Human TNIK consists of serine–threonine kinase and scaffold domains2146. TNIK interacts directly with TCF4 and β-catenin, and regulates Wnt signalling. TNIK phosphorylates TCF4 and regulates its transcriptional activity. TNIK was essential for full activation of Wnt signalling, and colorectal cancer cells were highly dependent on TNIK for growth.

Subsequent lead optimization resulted in the identification of NCB-0846 [cis-4-(2-(3H-benzo[d]imidazol-5-ylamino)quinazolin-8-yloxy)cyclohexanol] (left). NCB-0846 showed inhibitory activity against TNIK with an half-maximal inhibitory concentration (IC50) value of 21 nM, but its diastereomer (named NCB-0970) having the opposite configuration at the terminal hydroxyl group (right) showed 13-fold lower TNIK-inhibitory activity (IC50=272 nM). The crystal structure of the TNIK kinase domain (TNIK-KD) bound to either NCB-0846 or Compound 9 was determined at 2.9 or 2.4 Å resolution, respectively. The apo (unbound) and NCB-0846-bound TNIK-KD structures were almost completely superposable. NCB-0846 binds to the ATP-binding site in a 16-membered ring cyclic conformation by forming an intramolecular hydrogen bond between the benzimidazole N3 and the cyclohexanol O4. NCB-0846 interacts with the hinge region of TNIK-KD by forming two hydrogen bonds with the backbone carbonyl and amide groups of Cys108. In addition, the terminal hydroxyl group of the cyclohexanol forms another hydrogen bond with the main-chain carbonyl group of Gln157. This interaction with Gln157 is probably responsible for the potency of NCB-0846, because the diastereomer with the opposite configuration at this hydroxyl group (NCB-0970) showed impaired activity. Overall, the apo and NCB-0846-bound TNIK-KDs both adopt an inactive conformation. The RS2 (Phe172) and RS3 (Leu73) residues in the hydrophobic R-spine29 are not correctly assembled, and the salt bridge between Lys54 of β3 and Glu69 of the αC-helix is disrupted in these structures.

>GSGADEIDLSALRDPAGIFELVELVGNGTYGQVYKGRHVKTGQLAAIKVMDVTGDEEEEIKQEINMLKKYSHHRNIATYYGAFIKKNPPGMDDQLWLVMEFCGAGSVTDLIKNTKGNTLKEEWIAYICREILRGLSHLHQHKVIHRDIKGQNVLLTENAEVKLVDFGVSAQLDRTVGRRNTFIGTPYWMAPEVIACDENPDATYDFKSDLWSLGITAIEMAEGAPPLCDMHPMRALFLIPRNPAPRLKSKKWSKKFQSFIESCLVKNHSQRPATEQLMKHPFIRDQPNERQVRIQLKDHIDRTKKKRG[3x]> YGKPGPEGPEGPKG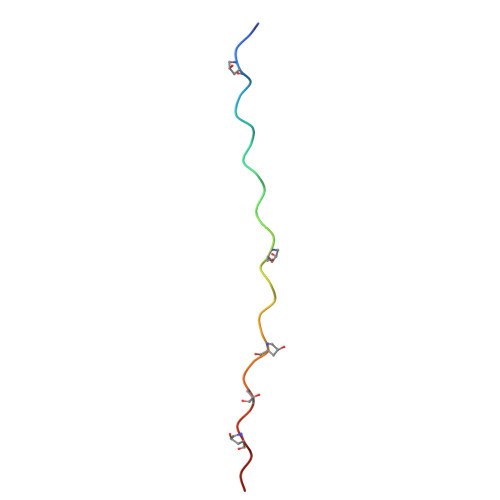KPGPKGKPGKPGKPGKA> MQPFDSGHDDLVHDVVYDFYGRHVATCSSDQHIKVFKLDKDTSNWELSDSWRAHDSSIVAIDWASPEYGRIIASASYDKTVKLWEEDPDQEECSGRRWNKLCTLN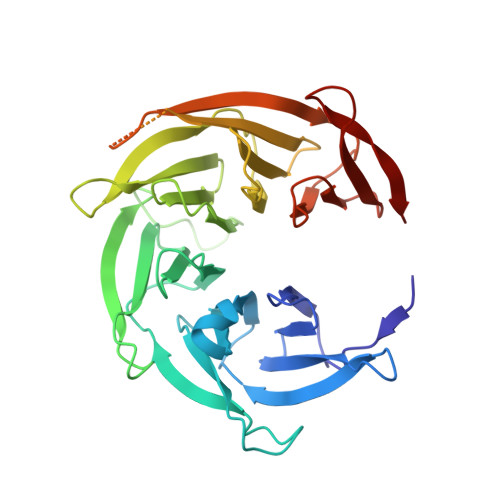DSKGSLYSVKFAPAHLGLKLACLGNDGILRLYDALEPSDLRSWTLTSEMKVLSIPPANHLQSDFCLSWCPSRFSPEKLAVSALEQAIIYQRGKDGKLHVAAKLPGHKSLIRSISWAPSIGRWYQLIATGCKDGRIRIFKITEKLSPLASEESLTNSNMFDNSADVDMDAQGRSDSNTEEKAELQSNLQVELLSEHDDHNGEVWSVSWNLTGTILSSAGDDGKVRLWKATYSNEFKCMSVITAQQ>GLDVAISQNGFFRLVDSNGSVFYSRNGQFKLDENRNLVNMQGMQLTGYPATGTPPTIQQGANPAPITIPNTLMAAKSTTTASMQINLNSTDPVPSKTPFSVSDADSYNKKGTVTVYDSQGNAHDMNVYFVKTKDNEWAVYTHDSSDPAATAPTTASTTLKFNENGILESGGTVNITTGTINGATAATFSLSFLNSMQQNTGANNIVATNQNGYKPGDLVSYQINNDGTVVGNYSNE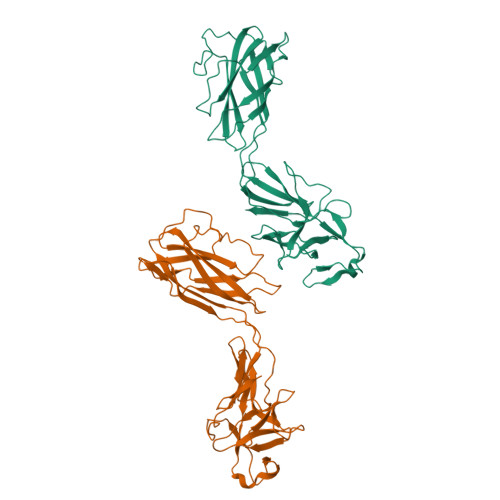QEQVLGQIVLANFANNEGLASQGDNVWAATQASGVALLGTAGSGNFGKLTNGALEASNVDLSK[2x]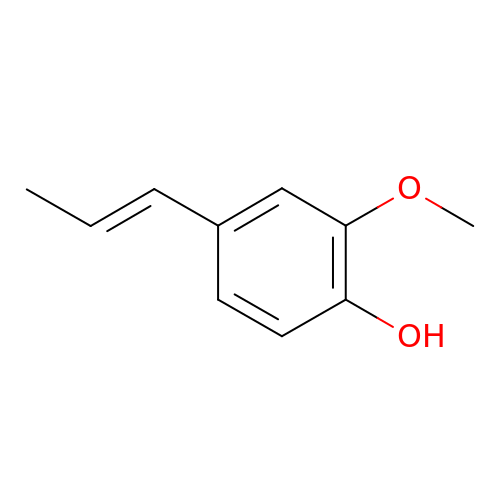2-methoxy-4-[(1E)-prop-1-en-1-yl]phenol | C10 H12 O2 | BJIOGJUNALELMI-ONEGZZNKSA-N>[2x]MKLKSFGVFGNPIKHSKSPLIHNACFLTFQKELRFLGHYHPILLPLESHIKSEFLHLGLSGANVTLPFKERAFQVCDKIKGIALECGAVNTLVLENDELVGYNTDALGFYLSLKQKNYQNALILGAGGSAKALACELKKQGLQVSVL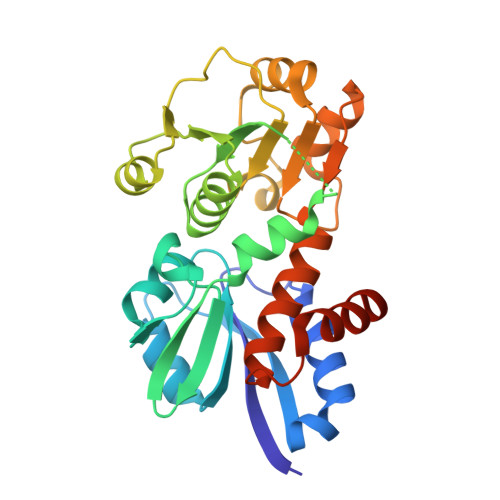NRSSRGLDFFQRLGCDCFMEPPKSAFDLIINATSASLHNELPLNKEVLKGYFKEGKLAYDLAYGFLTPFLSLAKELKTPFQDGKDMLIYNAALSFEKFSASQIPYSKAFEVMRSVFLEHHHHHH>GAHMFKIPGFGKAAANHTPPDMTNMDTRTRHLKVSNCPNNSYALANVAAVSPNDFPNNIYIIIDNLFVFTTRHSNDIPPGTIGFNGNQRTWGGWSLNQDVQAKAFDLFKYSGKQSYLGSIDIDISFRARGKAVSTVFDQDELAKQFVRCYESQIFSPTQYLIMEFQGHFFDLKIRNVQAIDLGDIEPTSAVATGIETKGILTKQTQINFFKGRDGLVNLKSSNSLRPRSNAVIRPDFKFEDLGVGGLDKEFTKIFRRAFASRIFPPSVIEKLGISHVKGLLLYGPPGTGKTLIARKIGTMLNAKEPKIVNGPEILSKYVGSSEENIRNLFKDAEAEYRAKGEESSLHIIIFDELDSVFKQRGSRGDGTGVGDNVVNQLLAKMDGVDQLNNILVIGMTNRKDLIDSALLRPGRFEVQVEIHLPDEKGRLQIFDIQTKKMRENNMMSDDVNLAELAALTKNFSGAEIEGLVKSASSFAINKTVNIGKGATKLNTKDIAKLKVTREDFLNALNDVTPAFGISEEDLKTCVEGGMMLYSERVNSI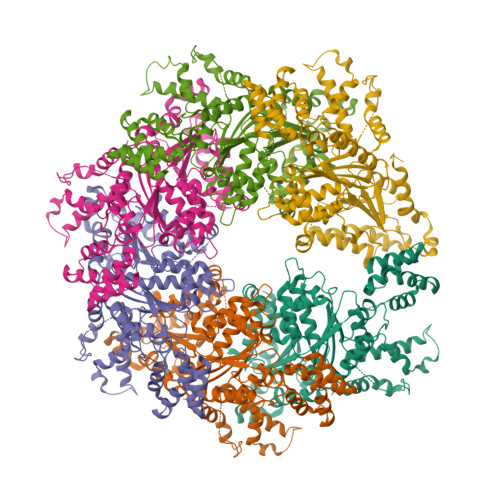LKNGARYVRQVRESDKSRLVSLLIHGPAGSGKTALAAEIALKSGFPFIRLISPNELSGMSESAKIAYIDNTFRDAYKSPLNILVIDSLETLVDWVPIGPRFSNNILQMLKVALKRKPPQDRRLLIMTTTSAYSVLQQMDILSCFDNEIAVPNMTNLDELNNVMIESNFLDDAGRVKVINELSRSCPNFNVGIKKTLTNIETARHDEDPVNELVELMTQSA[6x]>[2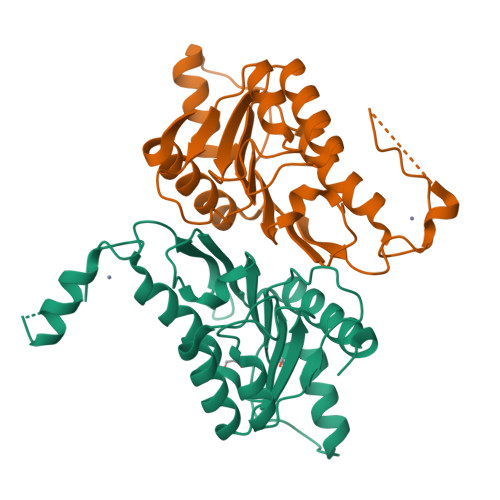x]GPGHMELRSKREKASRVHEVIIFNELGEICAAVHMRNSSMGSQKPQVSPCCNTHCSLRNVAKIVEQIDRAVYSIDLAIYTFTSLFLADSIKRALQRGVIIRIISDGEMVYSKGSQISMLAQLGVPVRVPITTNLMHNAFCIIDGFERVEEIRLLRKLKFMRPCYSIVISGSVNWTALGLGGNWENCIITADDKLTATFQAEFQRMWRAFAKTEGSQIQLK> SDQEPLYPVQVSSADARLMVFDKTEGTWRLLCSSRSNARVAGLSCEEMGFLRALTHSELDVRTAGANGTSGFFCVDEGRLPHTQRLLEVISVCDCPRGRFLAAICQDCGRRKLPVDRIVGGRDTSLGRWPWQVSLRYDGAHLCGGSLLSGDWVLTAAHCFPERNRVLSRWRVFAGAVAQASPHGLQLGVQAVVYHGGYLPFRDPNSEENSNDIALVHLSSPLPLTEYIQPVCLPAAGQALVDGKICTVTGWGNTQYYGQQAGVLQEARVPIISNDVCNGADFYGNQIKPKMFCAGYPEGGIDACQGDSGGPFVCEDSISRTPRWRLCGIVSWGTGCALAQKPGVYTKV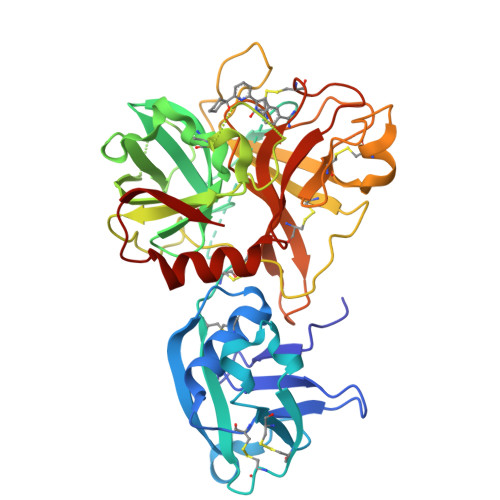SDFREWIFQAIKTHSEASGMVTQL> GPRFLKVKNWETDVVLTDTLHLKSTLETGCTEHICMGSIMLPSQHTRKPEDVRTKDQLFPLAKEFLDQYYSSIKRFGSKAHMDRLEEVNKEIESTSTYQLKDTELIYGAKHAWRNASRCVGRIQWSKLQVFDARDCTTAHGMFNYICNHVKYATNKGNLRSAITIFPQRTDGKHDFRVWNSQLIRYAGYKQPDGSTLGDPANVQFTEICIQQGWKAPRGRFDVLPLLLQANGNDPELFQIPPELVLEVPIRHPKFDWFKDLGLKWYGLPAVSNMLLEIGGLEFSACPFSGWYMGTEIGVRDYCDNSRYNILEEVAKKMDLDMRKTSSLWKDQALVEINIAVLYSFQSDKVTIVDHHSATESFIKHMENEYRCR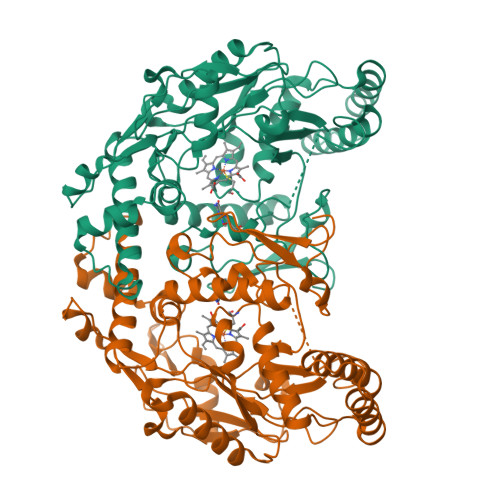GGCPADWVWIVPPMSGSITPVFHQEMLNYRLTPSFEYQPDPWNTHVW>MGFYSMPRYFQNMPQVGKPLKKADAANEEQLKKIEEEIHQLIKE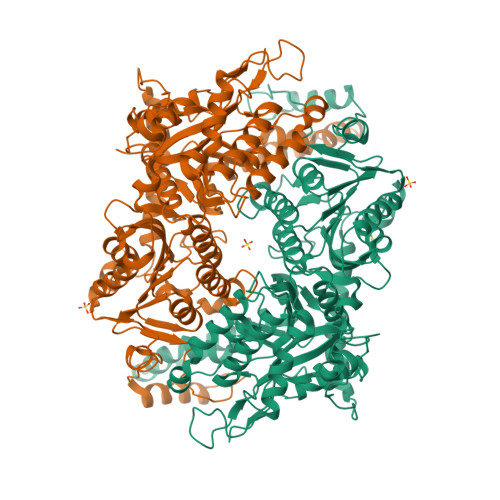AQEAGKADADVNKRGELTALQRIEKLVEPGSWRPLNTLFNPQGNKNGSVAIVKGLGRVNGKWCVVVASDNKKLAGAWVPGQAECLLRASDTAKTLHVPLVYVLNCSGVKFDEQEKVYPNRRGGGTPFFRNAELNQLGIPVIVGIYGTNPAGGGYHSISPTVIIAHEKANMAVGGAGIMGGMNPKGHVDLEYANEIADMVDRTGKTEPPGAVDIHYTETGFMREVYASEEGVLEGIKKYVGMLPKYDPEFFRVDDPKAPAFPADDLYSMVPLNDKRAYDIYNVIARLFDNSELHEYKKGYGPEMVTGLAKVNGLLVGVVANVQGLLMNYPEYKAAGSVGIGGKLYRQGLVKMNEFVTLCARDRLPIVWIQDTTGIDVGNDAEKAELLGLGQSLIYSIQTSHIPQFEITLRKGTAAAHYVLGGPQGNDTNAFSIGTAATEIAVMNGETAATAMYSRRLAKDRKAGKDLQPTIDKMNNLIQAFYTKSRPKVCAELGLVDEIVDMNKIRGYVEAFTEAAYQNPESICPFHQMILPRAIREFETFVKK[2x]> MAAKPVLYYFNGRGKMESIRWLLAAAGVEFEEVFLETREQYEKLLQSGILMFQQVPMVEIDGMKLVQTRAILNYIAGKYNLYGKDLKERALIDMYVGGTDDLMGFLLSFPFLSAEDKVKQCAFVVEKATSRYFPAYEKVLKDHGQDFLVGNRLSWADIHLLEAILMVE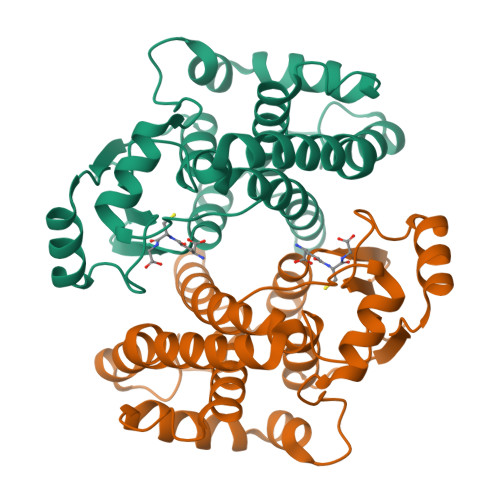EKKSDALSGFPLLQAFKKRISSIPTIKKFLAPGSKRKPISDDKYVETVRRVLRMYYDVKPH methyl 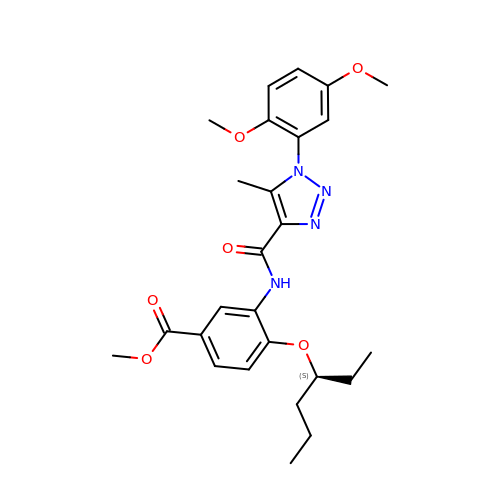3-{[(1P)-1-(2,5-dimethoxyphenyl)-5-methyl-1H-1,2,3-triazole-4-carbonyl]amino}-4-{[(3S)-hexan-3-yl]oxy}benzoate | C26 H32 N4 O6 | BBIKGMAYADRVGI-SFHVURJKSA-N methyl 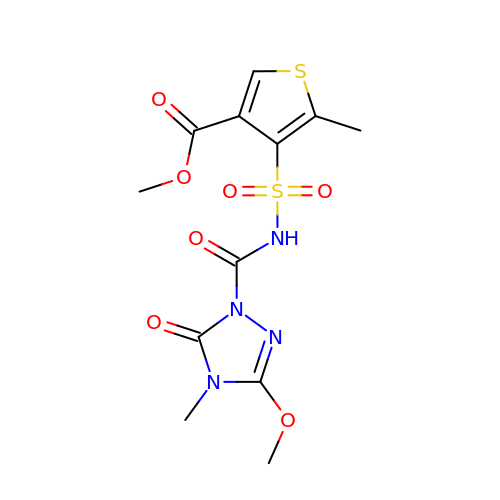4-[(3-methoxy-4-methyl-5-oxidanylidene-1,2,4-triazol-1-yl)carbonylsulfamoyl]-5-methyl-thiophene-3-carboxylate | C12 H14 N4 O7 S2 | XSKZXGDFSCCXQX-UHFFFAOYSA-N> MTWPLPDRLSINSLSGTPAVDLS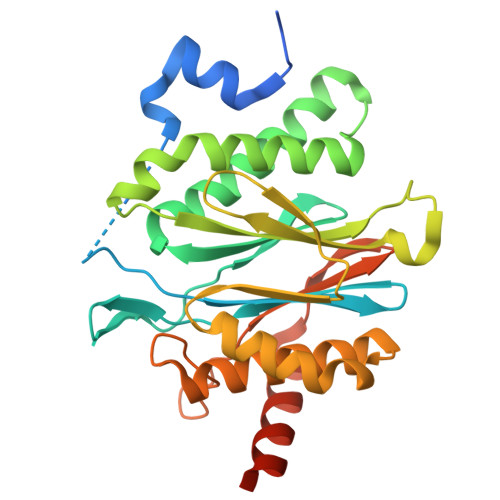SFTDFLRRQAPELLPASISGGAPLAGGDAQLPHGATIVALKYPGGVVMAGDRRSTQGNMISGRDVRKVYITDDYTATGIAGTAAVAVEFARLYAVELEHYEKLEGVPLTFAGKINRLAIMVRGNLAAAMQGLLALPLLAGYDIHASDPQSAGRIVSFDAAGGWNIEEEGYQAVGSGSLFAKSSMKKLYSQVTDGDSGLRVAVEALYDAADDDSATGGPDLVRGIFPTAVIIDADGAVDVPESRIAELARAIIESRSGADTFGSDGGEK> MANEPQKSDDNGQAAEAVVTDDEIVLQDQQLKTIEDEQKSVPLVATLAPFSILCAEYDNETSAAFLSKATELSEVYGEIRYIRGDGNCFYRAILVGLIEIMLKDRARLEKFIASSRDWTRTLVELGFPDWTCTDFCDFFIEFLEKIHSGVHTEEAVYTILNDDGSANYILMFFRLITSAFLKQNSEEYAPFIDEGMTVAQYCEQEIEPMWKDADHLA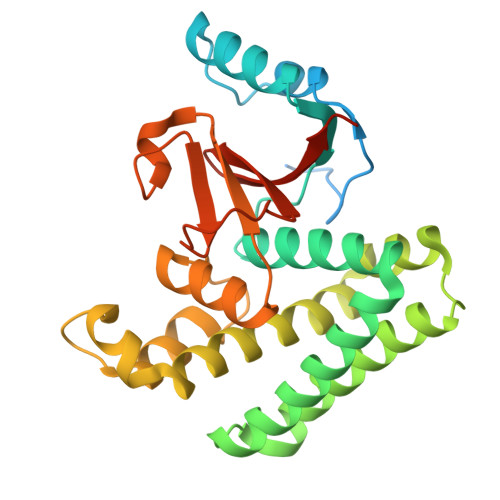INSLIKAAGTRVRIEYMDRTAAPNGGWHYDIPSDDQQIAPEITLLYRPGHYDVIYKKDSTEASEIEN> GPNSDVYAQEKQDFVQHFSQIVRVLTEDEMGHPEIGDAIARLKEVLEYNAIGGKYNRGLTVVVAFRELVEPRKQDADSLQRAWTVGWCVELLQAFFLVADDIMDSSLTRRGQICWYQKPGVGLDAINDANLLEACIYRLLKLYCREQPYYLNLIELFLQSSYQTEIGQTLDLLTAPQGNVDLVRFTEKRYKSIVKYKTAFYSFYLPIAAAMYMAGIDGEKEHANAKKILLEMGEFFQIQDDYLDLFGDPSVTGKIGTDIQDNKCSWLVVQCLQRATPEQYQILKEN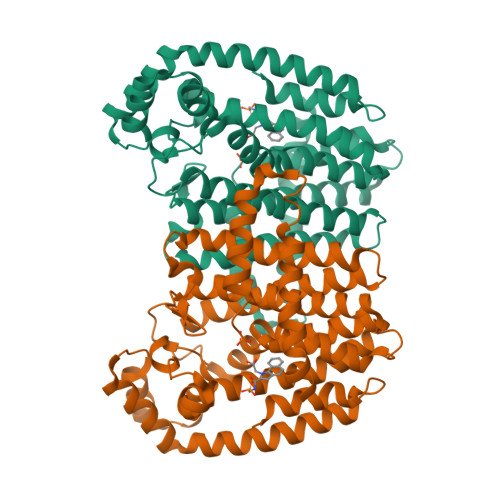YGQKEAEKVARVKALYEELDLPAVFLQYEEDSYSHIMALIEQYAAPLPPAVFLGLARKIYKRRK> DLTVKEKEELIEEWQPEPLVPPVPKDHPALNYNIVSGPPSHKTVVNGKECINFASFNFLGLLDNPRVKAAALASLKKYGVGTCGPRGFYGTFDVHLDLEDRLAKFMKTEEAIIYSYGFATIASAIPAYSKRGDIVFVDRAACFAIQKGLQASRSDIKLFKHNDMADLERLLKEQEIEDQKNPRKARVTRRFIVVEGLYMNTGTICPLPELVKLKYKYKARIFLEESLSFGVLGEHGRGVTEHYGINIDDIDLISANMENALASIGGFCCGRSFVIDHQRLSGQGYCFSASLPPLLAAAAIEALNIMEENPGIFAVLKEKCGQIHKALQGISGLKVVGESLSPAFHLQLEESTGSREQDVRLLQEIVDQCMNRSIALTQARYLEKEEKCLPPPSIRVVVTVEQTEEELERAASTIKEVAQAVLL;> MRPEPGGCCCRRTVRANGCVANGEVRNGYVRSSAAAAAAAAAGQIHHVTQNGGLYKRPFNEAFEETPMLVAVLTYVGYGVLTLFGYLRDFLRYWRIEKCHHATEREEQKDFVSLYQDFENFYTRNLYMRIRDNWNRPICSVPGARVDIMERQSHDYNWSFKYTGNIIKGVINMGSYNYLGFARNTGSCQ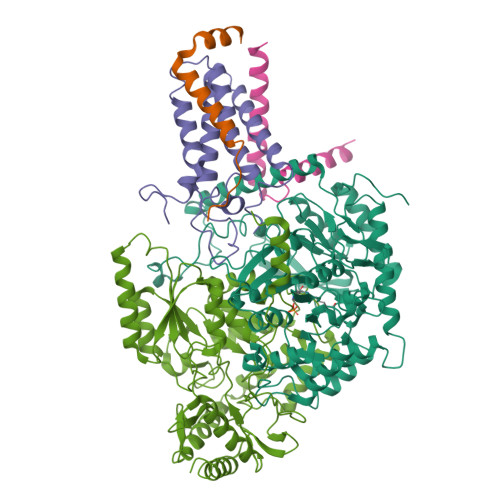EAAAKVLEEYGAGVCSTRQEIGNLDKHEELEELVARFLGVEAAMAYGMGFATNSMNIPALVGKGCLILSDELNHASLVLGARLSGATIRIFKHNNMQSLEKLLKDAIVYGQPRTRRPWKKILILVEGIYSMEGSIVRLPEVIALKKKYKAYLYLDEAHSIGALGPTGRGVVEYFGLDPEDVDVMMGTFTKSFGASGGYIGGKKELIDYLRTHSHSAVYATSLSPPVVEQIITSMKCIMGQDGTSLGKECVQQLAENTRYFRRRLKEMGFIIYGNEDSPVVPLMLYMPAKIGAFGREMLKRNIGVVVVGFPATPIIESRARFCLSAAHTKEILDTALKEIDEVGDLLQLKYSRHRLVPLLDRPFDETTYEETED;> MADYKDDDDKSGPDEVDASGRMAGMALARAWKQMSWFYYQYLLVTALYMLEPWERTVFNSMLVSIVGMALYTGYVFMPQHIMAILHYFEIVQ;> MVGTAHSEVNPNTRVMNSRGIWLSYVLAIGLLHIVLLSIPFVSVPVVWTLTNLIHNMGMYIFLHTVKGTPFETPDQGKARLLTHWEQMDYGVQFTASRKFLTITPIVLYFLTSFYTKYDQIHFVLNTVSLMSVLIPKLPQLHGVRIFGINKY;> MATATEQWVLVEMVQALYEAPAYHLILEGILILWIIRLLFSKTYKLQERS>GSHMASELNEHRATLFNKNVPSRAVKRVTAITKVEREAVLVCELPSFDVTDVEFDLFRARESTDKPLDVAAAIAYRLLLGSGLPQKFGCSDEVLLNFILQCRKKYRNVPYHNFYHVVDVCQTIHTFLYRGNVYEKLTELECFVLLITALVHDLDHMGLNNSFYLKTESPLGILSSASGNT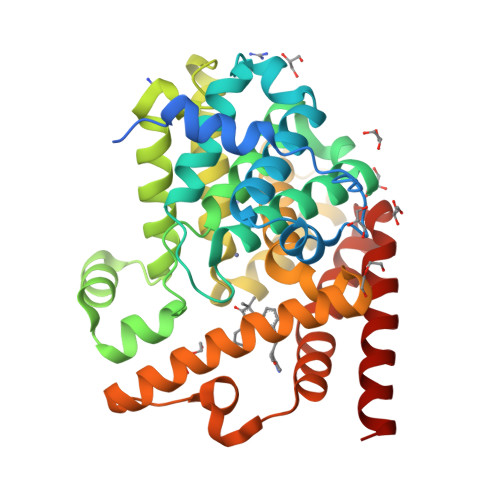SVLEVHHCNLAVEILSDPESDVFDGLEGAERTLAFRSMIDCVLATDMAKHGSALEAFLASAADQSSDEAAFHRMTMEIILKAGDISNVTKPFDISRQWAMAVTEEFYRQGDMEKERGVEVLPMFDRSKNMELAKGQIGFIDFVAAPFFQKIVDACLQGMQWTVDRIKSNRAQWERVLETR[2x]> MDEYSELSGIVDPRVLVTTSRDPSSRLMAFSKEIRLMFPTAIRLNRGNLILPDLVMSAQRERLSDIILLHEHRGTPTAITISHFPHGPTLMASLHNVVLRADIPKSIKGTVSESYPHLIFEGFRTPLGQRVVKILKHLFPPRDPTNNAKSGNRVITFVNQDDCIEVRHHVYVRTNYNSVELSEVGPRFTMRPFSITMGTLE;> MDADVERAEQDVRRDLFDDLSEHEDSEDALSDASAGDPKSRKSAHERRQAKIAEQIRKLEAELVAKRAWTLAGEATAADRPVNSLLGEDMEFDHVGKPVPVVTEEVSESIEELIKRRILAGEFDEV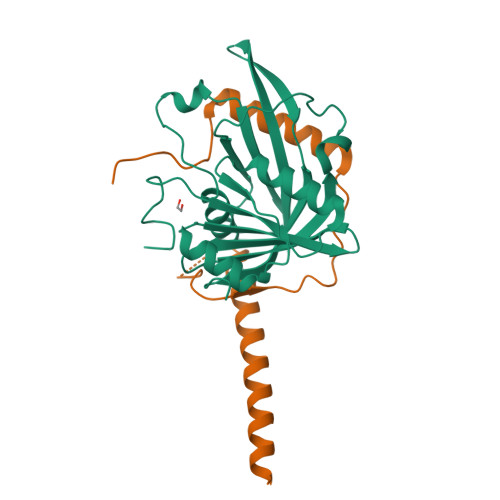LRRRP>MAANPYERGPNPTDALLEARSGPFSV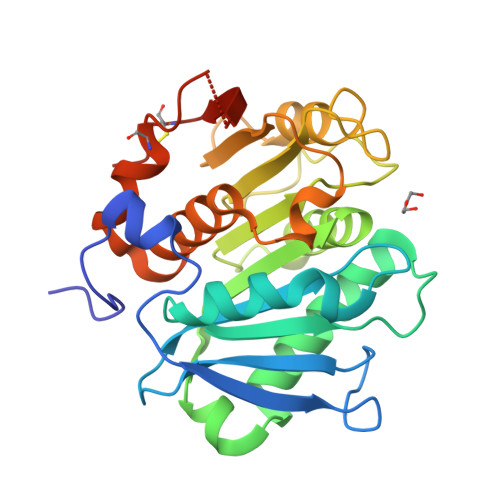SEENVSRLSASGFGGGTIYYPRESNTYGAVAISPGYTGTEASIAWLGERIASHGFVVITIDTITTLDQPDSRAEQLNAALNHMINRASSTVRSRIDSSRLAVMGHSMGGGGTLRLASQRPDLKAAIPLTPWHLNKNWSSVTVPTLIIGADLDTIAPVATHAKPFYNSLPSSISKAYLELDGATHFAPNIPNKIIGKYSVAWLKWFVDNDTRYTQFLCPGPRDGLFGEVEEYRSTCPFLEHHHHHH[6x]>M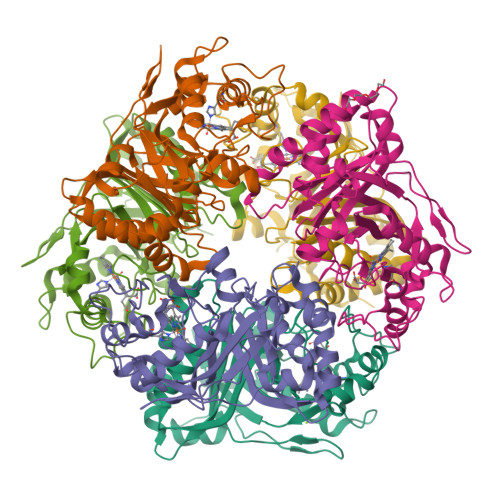GGEVEEPEPQMVLSPLTSAAIFLVVTIDSGGEDTVRDLLSDVASLERAVGFRAQPDGRLSCVTGIGSEAWDRLFSGARPAGLHPFRELDGPVHRAVATPGDLLFHIRASRLDLCFALATEIMGRLRGAVTPQDEVHGFKYFDERDMLGFVDGTENPTGAAARRAVLVGAEDPAFAGGSYAVVQKYLHDIDAWEGLSVEAQERVIGRRKMTDVELSDDVKPADSHVALTSVTGPDGSDLEILRDNMPFGSVGREEFGTYFIGYARTPEVTETMLERMFLGTASAPHDRILDFSTAVTGSLFFTPAADFLEDLSARP[6x]> GSDELYRQSLEIISRYLREQATGAKDTKPMGRSGATSRKALETLRRVGDGVQRNHETAFQGMLRKLDIKNEDDVKSLSRVMIHVFSDGVTNWGRIVTLISFGAFVAKHLKTINQESCIEPLAESITDVLVRTKRDWLVKQRGW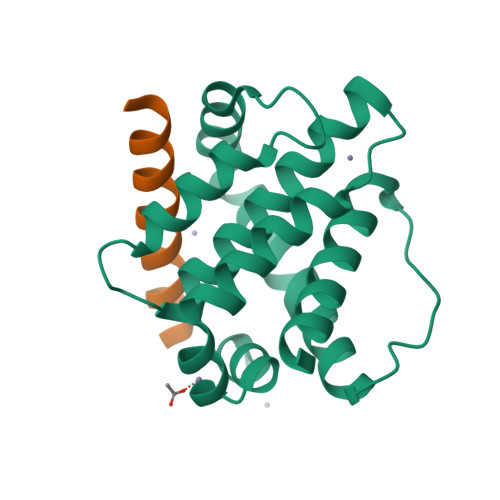DGFVEFFHVEDLEGG;> RPEIWIAQELRRIGDEENAYYR>SGRPMFSVFEEITRIVVKEMDAGGDMIAVRSLVDADRFRCFHLVGEKRTFFGCRHYTTGLTLMDILDTDGDKWLDELDSGLQGQKAEFQILDNVDSTGELIVRLPKEITISGSFQGFHHQKIKISENRISQQY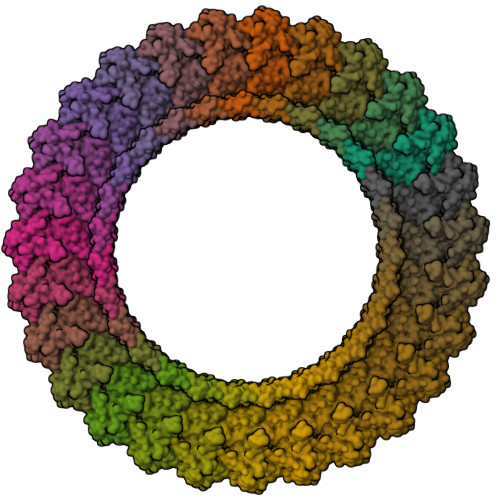LATLENRKLKRELPFSFRSINTRENLYLVTETLETVKEETLKSDRQYKFWSQISQGHLSYKHKGQREVTIPPNRVLSYRVKQLVFPNKETMNIHFRGKTKSFPEGKSLEVLFQ[27x]> MDDLTLRYFDAEMRYLREAGKAFAQAHPDRAAMLDLDKAGTPDPCVERLFEGFAFSMGRLRQKIDDDLPELTESLVSMLWPHYLRTIPSLSV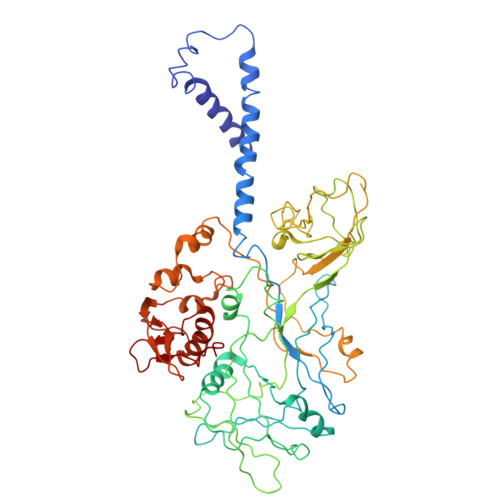VALTPRLSVMKMAETVPAGLEVTSRPVGPGNTVCRYRTTRAIPLNPLAVEKVVMTTEPDGRSVLKIGFACSELADWSQVDLHRLSLYLAAEAPVSSTLHLMMTKRLAALYLRLPGNDERIRIDGWFSPGGFAEEDRLWPKGDSAFSGYQLLLEYFTFREKFMFVHLNGLENVSLPAGISGFDLEVVLSQPWPADLPVTDDALCLHCVPVINLFTLEADPLIINGLESEYLLRPKRLQDGYTEIYSVDAVTGSGRTGSAEYVPFTSFRHRGGMLRHDAPERYYHTRVKRGVTGMYDTWLILGGQRWEADRMPERETLSLRITGTNGQLPRRALQSTLLDRCEQVLQAPVSVRNLCKPTLPVYPPTEDRFHWRVMSHLGTGFLNMLSSAEVLRGTLALYNWRDDELNHRRLDAILAVQHHRIQRFEKGFLLRGLDVEVTLDGNGFAGEGDIHLFGEMLNRFLALYADMNQFNQLTLIVQPEGKCIRWKENHNPRLPG Here we show that in addition to small-molecule antibiotics, Streptomyces produce and secrete antibacterial protein complexes that feature a large, degenerate repeat-containing polymorphic toxin protein. A cryo-electron microscopy structure of these particles reveals an extended stalk topped by a ringed crown comprising the toxin repeats scaffolding five lectin-tipped spokes, which led us to name them umbrella particles. Streptomyces coelicolor encodes three umbrella particles with distinct toxin and lectin composition. Each contains an amino-terminal twin arginine translocation (TAT) signal, two sets of four ALF repeats (ALF1–ALF8), two extended coiled-coil domains, and variable C-terminal and toxin domains.

We subsequently improved the resolvability of the regions constituting each spoke using local refinement, which produced reconstructions reaching up to 4.0 Å resolution. This process supported model building and provided a blueprint of the interactions underlying particle assembly. In line with our finding that UmbB1 interacts with individual ALF repeats, we were able to confidently model UmbB1 protomers in complex with ALF repeats at the base of each spoke. In spite of substantial variability in their sequences, ALF repeats bound UmbB1 at a stereotyped location, with residues in two of its short helical segments providing many key contacts. At several positions within this region that are highly conserved across each UmbB1-binding ALF repeat, ALF6 harboured dissimilar amino acids. To test the hypothesis that the amino acids in ALF6 at these positions prevent UmbB1 binding, we generated an ALF2 variant bearing the ALF6 residue at position four of its ALF repeat (ALF2(I4Q)). IP experiments demonstrated that this substitution abolished ALF2 binding to UmbB1. Owing to the conserved UmbA trypsin-like domain engagement by the N terminus of UmbB1, these configurations are anticipated to share similar overall structures. Finally, the Umb1 structure highlighted UmbB as a remarkable adaptor protein and keystone component of Umb toxin particles. That is, it interacts with five sequence divergent ALF repeats on one face and four different UmbA proteins on another.

> MRRRIPSRTPGSGAKQKSWFPRRSLQVLLSAGMLSGLLGTPAALAAEPAPLPANVRADIVGYWETGGAGLKAAAEQALLGGDEAIRKFLADAPSIQHDDNRIDAARMAMTGGSGLRQAAKDAIRLSPAELEKFLLYGYEEPLDDDHKVEIARLINLGGPGVREAGKAALQGTAEERELFLNSGQYTAQQDDNRVDVARLATTGGPNVQAAAKVALRGTPEDMVEFLEVGQFTARNRDQEHATIAELIKQAELAGKQADDARKTAEESSKKAVDASQLAKEAAQKAAEETEAAKDDSQKAAVKAKQAADAARAAADAAQEAIGSANAANRAARRAALAAAQTASAATAAAEAANKAYKAAIAAAGDEGKADEAKEAAKQARAAADAATKSGLAAENAGLASAAAATASTAAKSASSNARAAAGAAEEANQHADAAGVHSNEAALAAAEARRHADAADRAADRSSALAQRAATAAYGARDAANSAAEHANKAADYADESAAHAGDSAAYAATAKRNAQAAQEAAKTATAAVTKANEIFKLARETETANLETRTDAAIERARSMKSASETSITASATTQVEALALNDTATELAKEASRPDIDVQATAAKGRQLAMQAMKLLGPWHQEAAARALSGTDQDVLDYLRTRWKEANHNDIRQQIVDLSTQSPYASVRTAAAEALNGTPEQIEAFHTTGQYTAGSDDMKVDVARLANTGGPGVSQAAKTALADGTGKTLATFLQIGQYGERLSDEKVVTARLAETGSPEVQAAAKIALAGPPELLHEFVTTGQYMAKRKDDLADVHVNQVERLLAEGSLIAAEANEDAWRATEAAATAEGAAADAATAAEKAEASAAQAKQHAADADASADAATRSAADAAASAATARDAADRAAQDATAAENSAAEAAFSAAYARDSASKADDAADRARASALAAGKSADEAEAEAKEAWKTTRALAEKEAEEARRKAAEERKRQQEQAGEPKRVCIPHPTRETMIPIMPCAASPDDSMIMPGPVDPTIRAVVWELAGLNDIKACIDKPLSGNCVMAVVGVTPWGKFKLVSKLGNGLDAVKDARGARRTVACLTGAAHSFPAGTRVLMADGTRRSIEQIEAGDLVTATDPTTGETGARTVTRTIHTPDDRNFTDVALADGSTLTSTTHHPYWSQNDQTWKNAGDLEAGDTLRTPQNTAVVIAATHDWPGLQDAYDLTVDGFHSYYVSTGTTDVLVHNNDNPCPDWVSKAWKKLPKRKSGDPTSGYVFEADGTLVWDSVLTSGRSPLSEDISAFLKGSPDFPNFPGYADVAHHAEAKIAWEMRTKMGKGKKLHIVINTNYVCPKVSSPNSMGCKQAVPAILYEDQTLYVHYPGASDALELKGTAKR;> MANTSRTRQALMAIAVSVLAAGVTTLGVAHADNGDAVAAAAEMPQAVEDFSYPGAAKIQAETGAILKRGNGHMLMTSCDGSEDIQVMSRTGQKDFCFNVMAKPAYLTLEVPQAYGIWTSADPVKTTIKDTDGTATVINAPANDFTGYGEAGSTGEPTTLIELRVAG;> MFRMPRPIRATALSAAVLAGALASTPAQATVGDPTTDAKLDFTARLTIGTDYRSCSGALVDTQWVLTAASCFADDPNQPDTVAAGKPAQLTRATVGRADSNIANGYVREVVELVPHPERDMVLARLDKAIPDIAPVRLASDAPTAGTPLTAVGFGRTKDEWVPIQRHQGAFTVTSVTAGAVNVTGQGGDAICAGDTGGPLLQDKNGTLHLVGVNNRSMQGGCYGSETTSTDAIAAMSDADFVTQTVNRDLGTGNLSDLVASADFNSDGRTDVAAVLEDGSLHAFYAKPDGTLEYGRELWNDNTWSPMVQIIGGDFNSDGNGDIAAVRSDGTLNLYTGTATGILNKSKPMWHDTSWKTIKQVTRFKFNGRDGLVAQWGDGNLYGYYTGTDGTLTGTKVKMWPDATWGKTRLTGTADINADGRDDLTAVRDDGSLNWYAGNTKGGLDAARKLWPDNTWTPMKRIIGGDFNGDNKGDIAAVGGQSTLLLYTGTGTGTLNKGIAMRPASGSHHHHHHHH>[18x]GPLGSPEFMASGGGGCSASERLPPPFPGMDPESEGAAGGSEPEAGDSDTEGEDIFTGAAAATKPQSPKKTTSLFPIKNGSKENGIHEDQDQEPQDLFADATVELSLDSTQNNQKTMPGKTLTSHPPQEATNSPKPQPSYEELEEEQEDQFDLTVGITDPEKIGDGMNAYVAYKVTTQTSLPMFRSRQFAVKRRFSDFLGLYEKLSEKHSQNGFIVPPPPEKSLIGMTKVKVGKEDSSSAEFLEKRRAALERYLQRIVNHPTMLQDPDVREFLEKEELPRAVGTQALSGAGLLKMFNKATDAVSKMTIKMNESDIWFEEKLQEVECEEQRLRKLHAVVETLVNHRKELALNTALFAKSLAMLGSSEDNTALSRALSQLAEVEEKIEQLHQEQANNDFFLLAELLSDYIRLLAIVRAAFDQR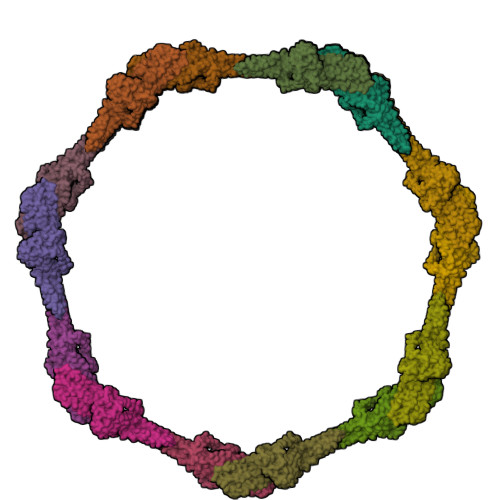MKTWQRWQDAQATLQKKRESEARLLWANKPDKLQQAKDEITEWESRVTQYERDFERISTVVRKEVTRFEKEKSKDFKNHVMKYLETLLHSQQQLAKYWEAFLPEAKAIS>MFPARLSLAVLFSVSPALAYFSGLGLGSERSIFRRDLNSTGDESNSTQWPAPLANGGKSWASAFKKAKATVTEMTVEELANITSGVIGLCSGVTGAVTRLGIPEFCLQDGPIGPRGVHGSSQFPAGLTVAATWDRTLMYARARGMGQEFHDQGVHLALAPVTGGPLGRTPLNGRGWEGTFADPYACGEASYLSVKGLTDAGVATVSKHWIAYEQETSRNLYIDIDGVSQADIQLPISSNVDDLTMHELYMWSFAEAVRAGTNHIMCSYNRINNTHSCSNAKGLNQLLKTELNFQGGVVSNWGGQWDSVPAAENGLDVAMPGKGFLGALGDFWGATLVELINNGTVSEDLVRDKAVRILTGYYYLGQDTNPPPPFVYNTIGAPTLNATSGYRNVRKPGTAELIKEIGSASVTLLKNTGSLPLKHPQRIAVLGNDATYNVLGPNACGLANSACDIDNLNGTLTTGGGSGSALSPYTITPLEALQKRAIEDNAEIAAVVANSNTTTGAEDAIAALLPDADVTFVFLNRYSEEGADAPDFSLGGDGDNLMDLAVTYSSNVVVVIHTTGVVDIEKWADNPNVTAILVAYLPGQEAGNSLVPVLYGDVAPSGKLPWTWGKSIDDYVPNGVVYTDAYSPQSNFTEGVFIDYRWFDKMGITPRYEFGFGLSYTTFTYSNLIVDHGRWAKDYSSVMETAEPFAEWDGTNS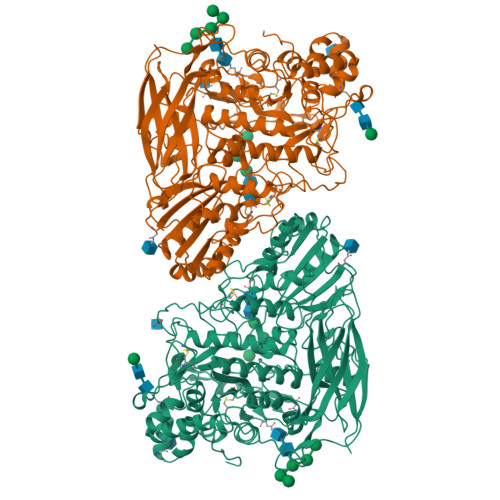LYDVIFTVFATITNTGNLTGSEVAQLYISIPGDNQPVRQLRGFDKIKDLPVGDSAVVTFPIRRKDVSSWSVVDQLWYVPNGDFLISVGGSSRDLPLNTTWTPHH[6x]> HHHHHHDITFRNIRFRYKPDSPVILDNINLSIKQGEVIGIVGRSGSGK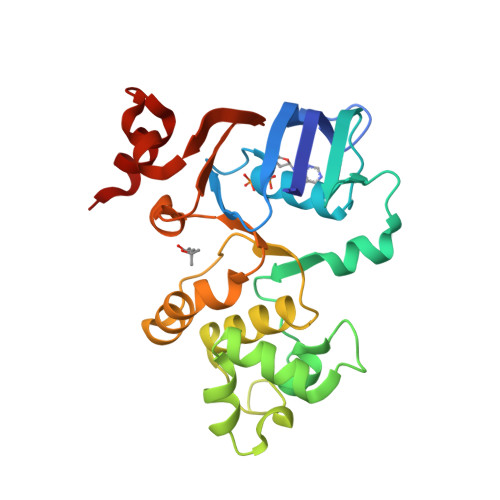STLTKLIQRFYIPENGQVLIDGHDLALADPNWLRRQVGVVLQDNVLLNRSIIDNISLANPGMSVEKVIYAAKLAGAHDFISELREGYNTIVGEQGAGLSGGQRQRIAIARALVNNPKILIFDEATSALDYESEHVIMRNMHKICKGRTVIIIAARLSTVKNADRIIVMEKGKIVEQGKHKELLSEPESLYSYLYQLQSD>[2x]GGGRKSITESFATAIHGLKVGHLTDRVIQRSKRMI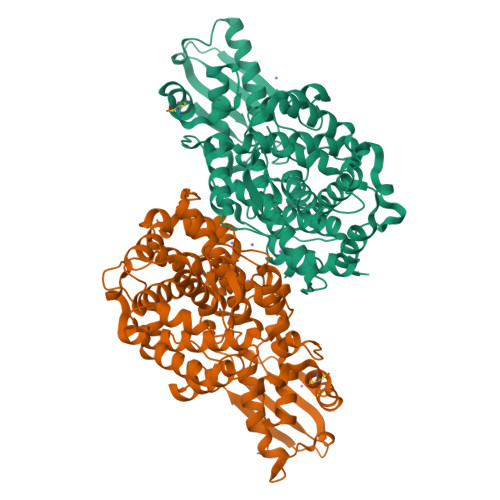LDTLGAGFLGTTTEVFHIASQYSKIYSSNISSTVWGQPDIRLPPTYAAFVNGVAIHSMDFDDTWHPATHPSGAVLPVLTALAEALPRSPKFSGLDLLLAFNVGIEVQGRLLHFAKEANDMPKRFHPPSVVGTLGSAAAASKFLGLSSTKCREALAIAVSHAGAPMANAATQTKPLHIGNAAKHGIEAAFLAMLGLQGNKQVLDLEAGFGAFYANYSPKVLPSIASYSWLLDQQDVAFKRFPAHLSTHWVADAAASVRKHLVAERALLPTDYIKRIVLRIPNVQYVNRPFPVSEHEARHSFQYVACAMLLDGGITVPSFHECQINRPQVRELLSKVELEYPPDNLPSFNILYCEISVTLKDGATFTDRSDTFYGHWRKPLSQEDLEEKFRANASKMLSWDTVESLIKIVKNLEDLEDCSVLTTLLKGP4-(BENZHYDRYLOXY)-1-[3-(1H-TETRAAZOL-5-YL)PROPYL]PIPERIDINE | C22 H27 N5 O | 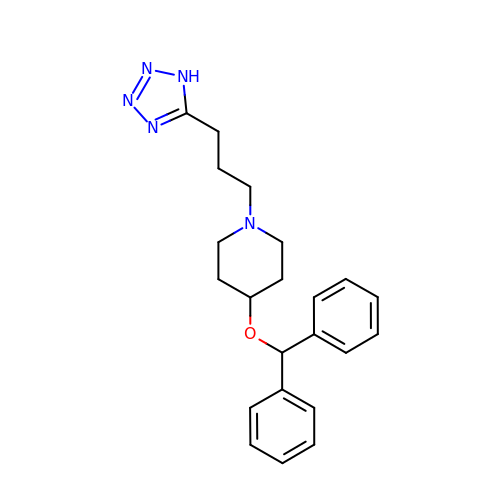TZQGXAHOROZEKN-UHFFFAOYSA-N> MQNEKLDHESVTQAMQPKDTPELRALYKSFEEESIIPLWTQLGDLMPIHPKSKAVPHVWKWSTLLRLARKSGELVPVGRGGERRALGLANPGLGGNAYISPTMYAGIQYLGPRETAPEHRHSQNAFRFVVEGEGVWTVVNGDPVRMSRGDLLLTPGWCFHGHMNDTDQPMAWIDGLDIPFSQQMDVGFFEFGSDRVTDYATPNFSRGERLWCHPGLRPLSGLQNTVASPIGAYRWEFTDRALTEQLLLEDEGQPATVAPGHAAIRYVNPTTGGDVMPTLRCEFHRLRAGTET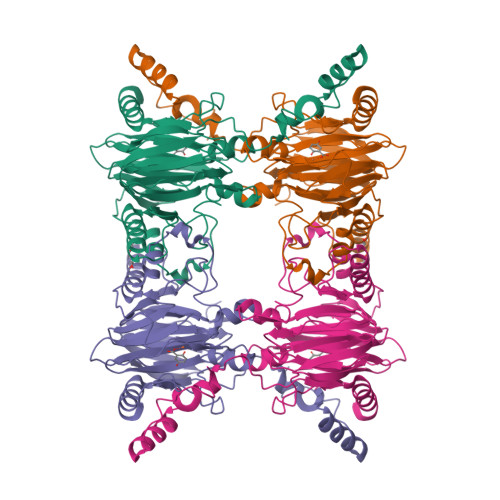ATRNEVGSTVFQVFEGAGAVVMNGETTKLEKGDMFVVPSWVPWSLQAETQFDLFRFSDAPIMEALSFMRTKIEGQ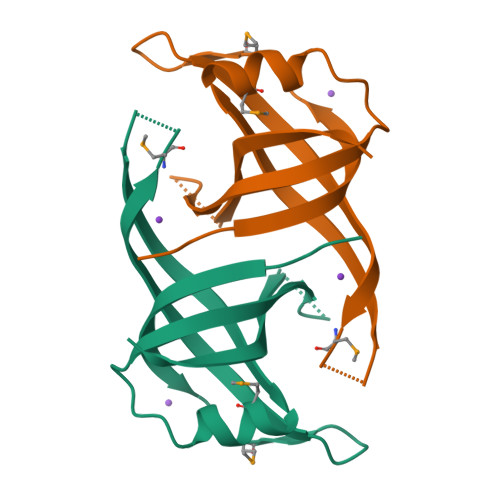> AINRLQLVATLVEREVMRYTPAGVPIVNCLLSYSGQAMEAQAARQVEFSIEALGAGKMASVLDRIAPGTVLECVGFLARKHRSSKALVFHISGLEHHHHHH> 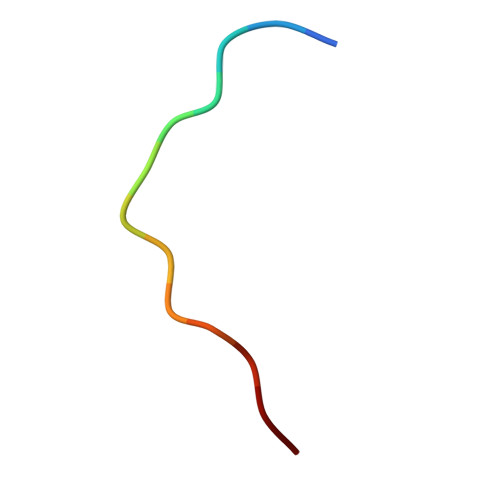SGATTATTTTSNS> MAETNFNYSKLLRNLVTEDNVLNEVVVSFLYQLFPRDLFVRAFSLLESA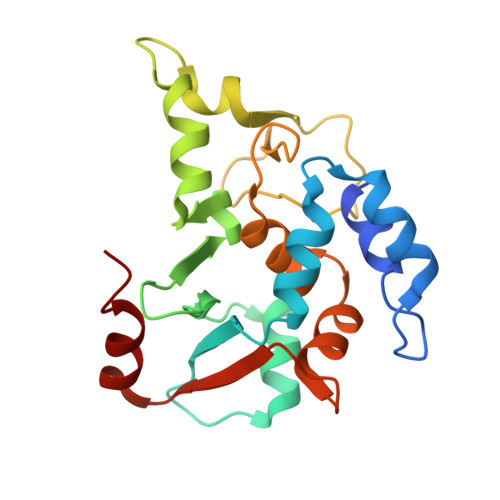DMFIYVWMPTPKEADELLESLYNGTPLYRPIVRPRGPDDRPVCVDLDHWFCSCTEFAATCRPHLVGDTPLSDALFRPTEAADPDDCFGMLAGLQHLRADPEKLMCEHLFAFAILLQTDLRVLRHFSTGPGAQVFVLGITSIDEWLKLHLNVV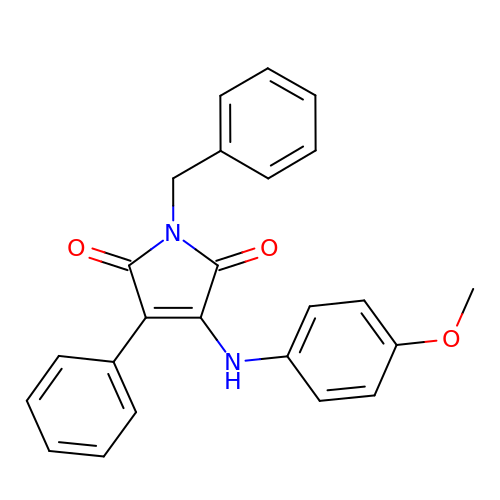1-BENZYL-3-(4-METHOXYPHENYLAMINO)-4-PHENYLPYRROLE-2,5-DIONE | C24 H20 N2 O3 | HLZMYWLMBBLASX-UHFFFAOYSA-N> MESLPVIAAPSMWTRPQIKDFKEKIQQDADSVITVGRGEVVTVRVPTHEEGSYLFWEFATDNYDIGFGVYFEWTDSPNTAVSVHVSESSDDDEEEEENIGCEEKAKKNANKPLLDEIVPVYRRDCHEEVYAGSHQYPGRGVYLLKFDNSYSLWRSKSVYYRVYYTR;> GPLQYKDLKIDIKTSPPPECINDALQAVDSQEVRDYCEKKGWIVNITSQVQTERNINR

ACBD3 is a Golgi resident protein involved in the maintenance of the Golgi structure and regulation of intracellular trafficking between the endoplasmic reticulum and the Golgi. However, in enterovirus-infected cells, the ACBD3 GOLD domain interacts preferentially with viral non-structural 3A proteins, which causes re-localization of ACBD3 to the sites of virus replication. In this study, we present a structural, biochemical, and biological characterization of the complexes composed of human ACBD3 and the 3A proteins of four representative enteroviruses. The crystal structures revealed the details of the ACBD3-3A interaction, the 3A-3A interaction causing the assembly of the ACBD3-3A heterotetramers, the interaction between the ACBD3-3A complex and the lipid bilayer, and the roles of these interactions in facilitation of enterovirus replication.

The first strategy was based on mutagenesis of selected surface-exposed hydrophobic residues of the 3A proteins to improve the solubility of the respective GOLD: 3A complexes and their capability to be crystallized at higher protein concentrations. This approach led to a successful crystallization of the GOLD: 3A/PV1 complex with an L24A point mutation within the PV1 3A protein. The overall structures of all solved GOLD: 3A complexes are highly similar to each other. This suggests that neither the L24A mutation in the GOLD: 3A/PV1 complex nor the fusion-protein strategy used for the GOLD: 3A/EVA71 complex affected the overall fold of the complexes. Analysis of the crystal structures of the GOLD: 3A complexes revealed that the 3A proteins formed either one of the crystal-packing contacts (as in the case of EVD68 and PV1) or contacts with the second 3A molecule when two GOLD: 3A complexes per asymmetric unit were present (as in the case of EVA71 and RVB14). For instance, the poliovirus 3A strand β23A/PV1 binds in the antiparallel orientation to the strand V402ACBD3-P408ACBD3 of ACBD3, while the aichivirus 3A strand β13A/AiV1 binds at the same position to the same strand of ACBD3, but in the parallel orientation. Superposition of the crystal structures of the enterovirus and kobuvirus 3A: GOLD complexes reveals that the enterovirus and kobuvirus 3A proteins bind to the same regions of the ACBD3 GOLD domain, nevertheless, the polypeptide chains of the enterovirus and kobuvirus 3A proteins have opposite polarities.> GPGGSMITVNEKEHILEQKYRPSTIDECILPAFDKETFKSITSKGKIPHIILHSPSPGTGKTTVAKALCHDVNADMMFVNGSDCK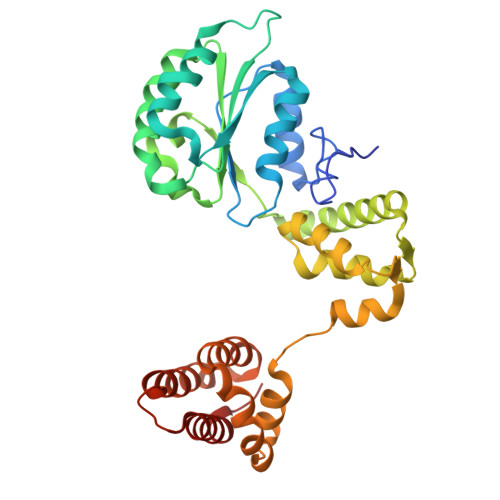IDFVRGPLTNFASAASFDGRQKVIVIDEFDRSGLAESQRHLRSFMEAYSSNCSIIITANNIDGIIKPLQSRCRVITFGQPTDEDKIEMMKQMIRRLTEICKHEGIAIADMKVVAALVKKNFPDFRKTIGELDSYSSKGVLDAGILSLVTNDRGAIDDVLESLKNKDVKQLRALAPKYAADYSWFVGKLAEEIYSRVTPQSIIRMYEIVGENNQYHGIAANTELHLAYLFIQLACEMQWK> GGGUUAUGUGUGCCCGGCAUGGGUGCAGUCUAUAGGGUGAGAGUCCCGAACUGUGAAGGCAGAAGUAACAGUUAGCCUAACGCAAGGGUGUCCGUGGCGACAUGGAAUCUGAAGGAAGCGGACGGCAAACCUUCGGUCUGAGGAACACGAACUUCAUAUGAGGCUAGGUAUCAAUGGAUGAGUUUGCAUAACAAAACAAAGUCCUUUCUGCCAAAGUUGGUACAGAGUAAAUGAAGCAGAUUGAUGAAGGGAAAGACUGCAUUCUUACCCGGGGAGGUCUGGAAACAGAAGUCAGC

The prototypical systems used to study sequential RNA assembly are group II introns, another class of highly-conserved self-splicing ribozymes of biomedical and bioengineering relevance. Group II introns are validated drug targets for antifungal antibiotics, potentially powerful vectors for genetic engineering, and the evolutionary ancestors of the catalytic RNA core of the eukaryotic spliceosome. Integrating single-particle electron cryomicroscopy (cryo-EM), image processing, in solution small-angle X-ray scattering (SAXS), EM-driven molecular dynamics (MD) simulations, structure-based mutagenesis, and enzymatic assays, we have visualized the sequential multidomain assembly of a self-splicing ribozyme of biomedical and bioengineering significance. Our work reveals a distinct dynamic interplay of helical subdomains in the ribozyme’s 5’-terminal scaffold, which acts as a gate to control the docking of 3’-terminal domains.

A Coulomb potential density map of the “partly open” state of D1-2 at 4.33 Å resolution. One conformation, hereafter referred to as the “partly open” state, displays a distinct orientation of ‘peripheral D1c’, which differs clearly from the “catalytic” state despite laterally flanking i1-i2 and D2. In the D1-2 dataset, we can observe complete density for D2 in the “partly open” state, but not in the “fully open” state. However, D2 is not stably bound to D1 in this state, but only transiently docks onto D1 by establishing the θ-θ’ interaction in the ‘partly open’ state. Importantly, the most highly-resolved maps show that, in the “partly open” conformation of both D1-2 and D1-3, hinge 1 residue A72 orients towards the core of the D1c helix, as in the “catalytic” state, but C116 bulges out of the helix, as in the “closed” state, and its solvent-exposed nucleobase remains disordered. Hinge 2 residues (A217 and A223-A224), instead, do not show major conformational changes between the two states in either construct. Furthermore, ‘angle A’ progressively increases from 65.8° for sub-state model 1 to 80.5° for sub-state model 20 for the D1-2 dataset, and from 66.9° for sub-state model 1 to 75.1° for sub-state model 20 for the D1-3 dataset, respectively. Finally, the ‘gate distance’ progressively increases from 33.8 Å for sub-state model 1 to 37.8 Å for sub-state model 20 for the D1-2 dataset, and from 34.6 Å for sub-state model 1 to 36.5 Å for sub-state model 20 for the D1-3 dataset, respectively. In line with these chemical probing data, here we show that θ-θ’ is not stably formed in the “open” conformations of D1-2, D1-3, and D1-4.>GMTTSKLEKTGLHVHEKIKHMVKNYGTMITGIPAEILGQNEAEISVGYVKKMGNMKENIAEVVRKSEMTQPTNSAGKASNEVCDLLLGTEGASEFEKSSYQVLSGDGSNLKGSLPNKNLLVRVEMDRFNAPQKYQKIKREEFNPETAEKNKIYLLEDQLVYLDIFGKVIDLGQTSDTCHRLFNAITTPFYQNYILYDEYIDPEESAEEAAMFEMGEIVKAKMKNIDCWTATHSFTIFVPESDSEDTRTLYPYQAYWTSHTLQQWFSGDKDEKLSRLGIDGYIEKLALLGTTTDSKIRSSIYGELFSPPGKEHVFCTGMN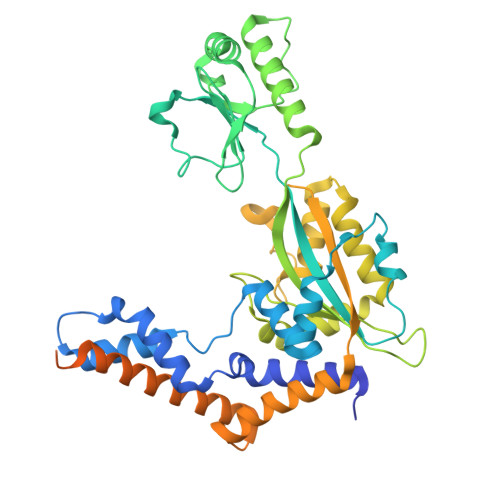EKFSPLRVKFKVTEVNPEIALQNLEEVQEFIDTNYPGENAKDQCELYKIKAQEAMTKQLEMRLLIEPTHRKESVTPYKEKNTQSFFSKNLDTTSRIDKMISSVITMENLKILAKEADTLSGKDREKLVEYFKTLPSEQLAEIKA[2x]>MKKEIQVQGVRYYVESEDDLVSVAHELAKMGYTVQQIANALGVSER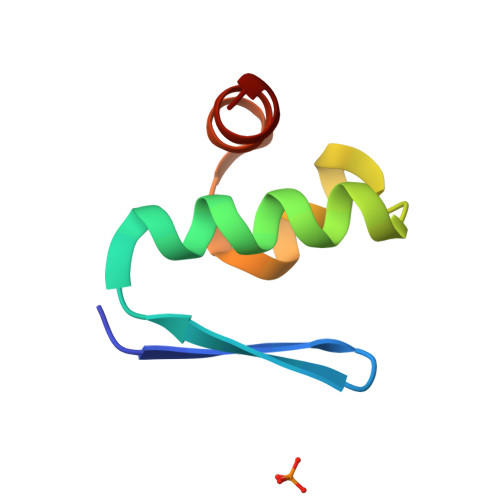KVRRYLESC[3x]> AKEIPEVLVDPRSRRRYVRGRFLGKGGFAKCFEISDADTKEVFAGKIVPKSLLLKPHQREKMSMEISIHRSLAHQHVVGFHGFFEDNDFVFVVLELCRRRSLLELHKRRKALTEPEARYYLRQIVLGCQYLHRNRVIHRDLKLGNLFLNEDLEVKIGDFGLATKVEYDGERKKVLCGTPNYIAPEVLSKKGHSFEVDVWSIGCIMYTLLVGKPPFETSCLKET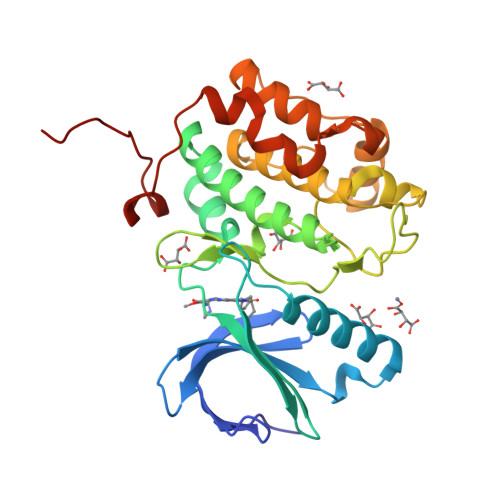YLRIKKNEYSIPKHINPVAASLIQKMLQTDPTARPTINELLNDEFFTSGYIPARLPITCLTIPPRFSIAPS>[2x]MADDQGCIEEQGVEDSANEDSVDAKPDRSSFVPSLFSKKKKNVTMRSIKTTRDRVPTYQYNMNFEKLGKCIIINNKNFDKVTGMGVRNGTDK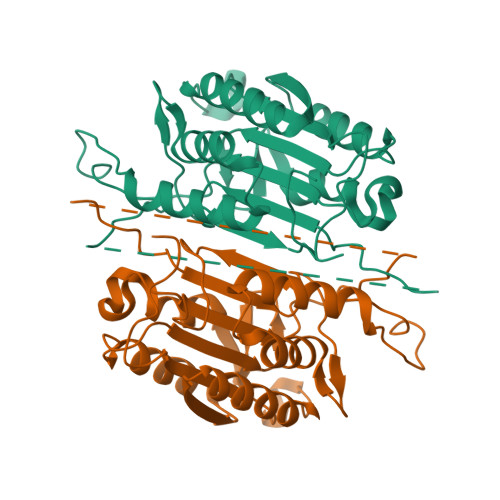DAEALFKCFRSLGFDVIVYNDCSCAKMQDLLKKASEEDHTNAACFACILLSHGEENVIYGKDGVTPIKDLTAHFRGDRCKTLLEKPKLFFIQACRGTELDDGIQADMSGPINDTDANPCYKIPVEADFLFAYSTVPGYYSWRSPGRGSWFVQALSSILEEHGKDLEIMQILTRVNDRVARHFESQSDDPHFHEKKQIPCVVSMLTKELYFSQLEHHHHHH> NAQPNLGRSTKATPDFPTHFPKSSIGIQNELAGLVVAMPANSAQKFGYVKSAQGDALFMLTKDMNQGSYQRPPSLQDGKNYQNWQTHTVELVSYPCEMDDKAAVETRKQAMLWLATHFTTHIDQSNHQPLAPIQSEDGRFVIEITNAKHVIAAGNGISAESQGQTITMTPSGQQATVG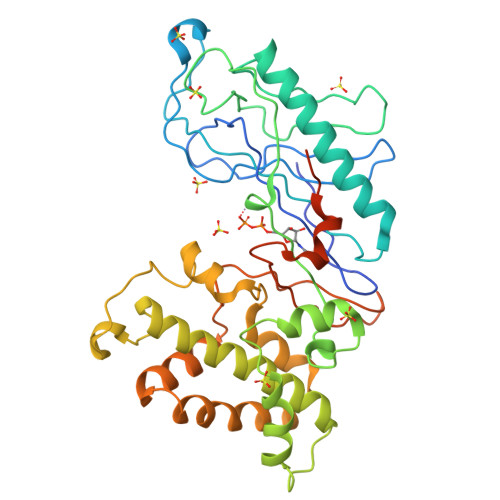VAAKGFGTSATPELRLLESAPWYQKSLKSQFASLTSAENLDDKELAANVFAYLTSIYLKTAELAKKFGIYINEWDPMSEQITPNANGLTDPKVKNAWEILPRTKPSKIVEILSKSDAKAVMKHIKPQLQSRYSESLSKNVFQYFQDGGEVAGHGINNATVGDKHSPELAILFEFRTVPNELQSYLPKTESTTKSEVKLLDQFDPMKRKTVIQQVESLV>[7x]APGQSKKKIFKPEELR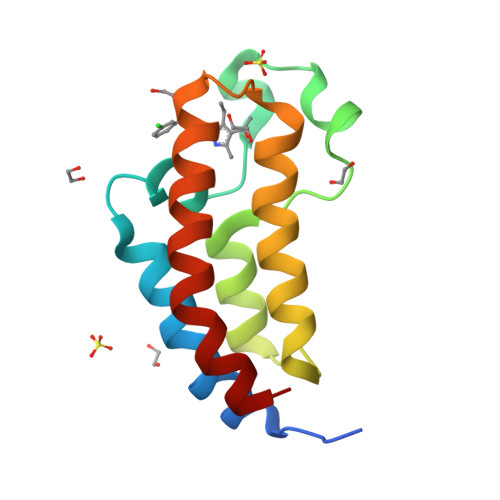QALMPTLEALYRQDPESLPFRQPVDPQLLGIPDYFDIVKSPMDLSTIKRKLDTGQYQEPWQYVDDIWLMFNNAWLYNRKTSRVYKYCSKLSEVFEQEIDPVMQSLG>[4x]MAYRICLIEGDGIGHEVIPAARRVLEATGLPLEFVEAEAGWETFER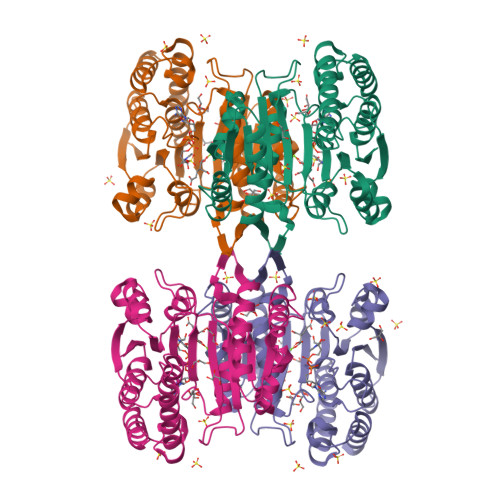RGTSVPEETVEKILSCHATLFGAATSPTRKVPGFFGAIRYLRRRLDLYANVRPAKSRPVPGSRPGVDLVIVRENTEGLYVEQERRYLDVAIADAVISKKASERIGRAALRIAEGRPRKTLHIAHKANVLPLTQGLFLDTVKEVAKDFPLVNVQDIIVDNCAMQLVMRPERFDVIVTTNLLGDILSDLAAGLVGGLGLAPSGNIGDTTAVFEPVHGSAPDIAGKGIANPTAAILSAAMMLDYLGEKEAAKRVEKAVDLVLERGPRTPDLGGDATTEAFTEAVVEALKSL> KVFERCELARTLKRLGMDGYRGISLANWMCLAKWESGYNTRA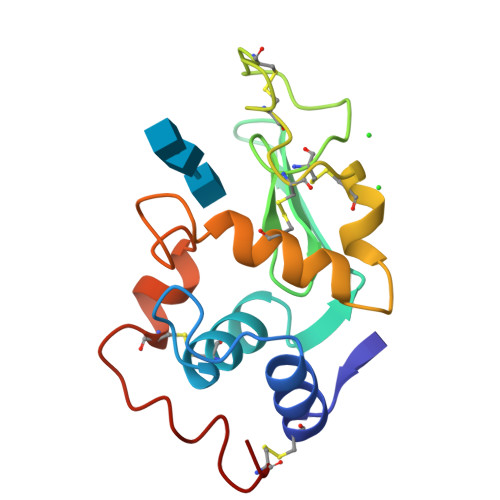TNYNAGDRSTDYGIFQINSRYWCNDGKTPGAVCRGDSCNACHLSCSALLQDNIADAVACAKRVVRDPQGIRAWVAWRNRCQNRDVRQYVQGCGV> MDKEIYCGSVPVSYFDPFDLFESLRPE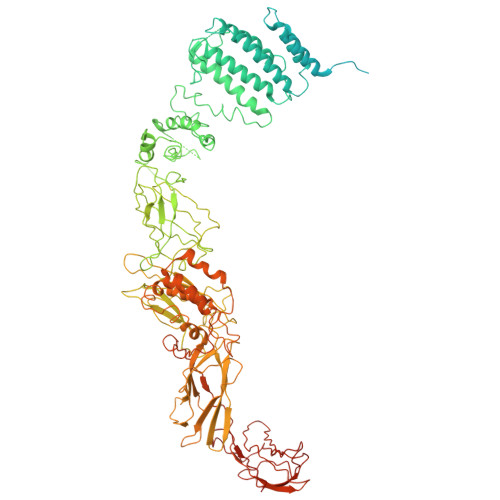FQQILPLDNIHWKAFDGTVRTVNRLPIELIPEGRGEADKSNDEQPFIRFLIVNCISIDQYRAKVRPLVRQWLPNLESVSSSTGEKMIYKPIILLYANSEVVDSNLFKSVSLMEKFGKDFPHVQTLEVRSVYRSPKERQEFWNQFSQKIKASVLSIFQKRLTHLQHSLANLQKGNNFEEQLLTREKLYELYVVFNILEDASLELQKIKKEILRRNMNMPDGKLQVPFESSSKSDESLGSIIIEGTLDKFQLHKYFFIRRLRLLKLEDQTLTAFVGAFQLIKNFIESISIEYRKSVRLLEFKHYFITSMLSYFEFENVSNPLLCEIKAELLMLKRDNWVQGVMATSGYRLMDKNYPNSDVKYKFDLLKETFVDETVFQENFLTLTKEILSLFNKCEGKRQRIVDILSIEIGLLYYQGKKYEEAVSLFLSCYEYYTQTNWNSIGLKILQVFIDSLSHCPKLDVLQIDGESVSASAVLTNAFLNILKLCKDNDSKEIWWKKFMDLQMKNNIHLMYPLDGLFEVTLNSKVHLARANVSAIEVNLKSYGFPEDISTKTMRLSLKNMGGDVIVFGASDFLLKKGENKLILECRDIMYGEFSLLSFEIIVEGITFVKEFPENQDEFIVVPEIYCKESTKVLVKQAHNLNLGEYALELKSVQSDALESLQVEVEVQKNIGNMKNLPVSFSMDEIQARKRYNTPFENVRLEYYLLDQITAFDLIIKTSFTKKNDQGTFGETKKVRIQCYLQLSVSVEDIFKKDIFFFKFLLNSSVREEPVILYSSELSAPDTRNDYNIRGDYIATTPALITFDGNESFINCYEITANNNFDSKDIFNLKVRYNTLKEQLDCFITDAVLIEGDVEWFILFEKWKTFWELEILKKLKYDYDAFKENRIIRLLKTSIDLNKTKSKIRNLCIEKAVLDKILICLNKVSRGIAVCNTDMDEYVRNLVPKQLTVPVQLPGFEQFFHVQFEQMETSHDALHDTIATIGNSLSYTVIVENLSGQWGQDVIDDGGYIFEILSSNEWLIHGQKRCAIKEKRKEFEVHLIPLKKGYLNFPRVEITNINGKSCRVDHSNAFESILIF> SRCTHLENRDFVTGTQGTTRVTLVLELGGCVTITAEGKPSMDVWLDAIYQENPAKTREYCLHAKLSDTKVAARCPTMGPATLAEEHQGGTVCKRDQSDRGWGNHCGLFGKGSIVACVKAACEAKKKATGHVYDANKIVYTVKVEPHTGDYVAANETHSGRKTASFTISSEKTILTMGEYGDVSLLCRVASGVDLAQTVILELDKTVEHLPTAWQVHRDWFNDLALPWKHEGAQNWNNAERLVEFGAPHAVKMDVYNLGDQTGVLLKALAGVPVAHIEGTKYHLKSGHVT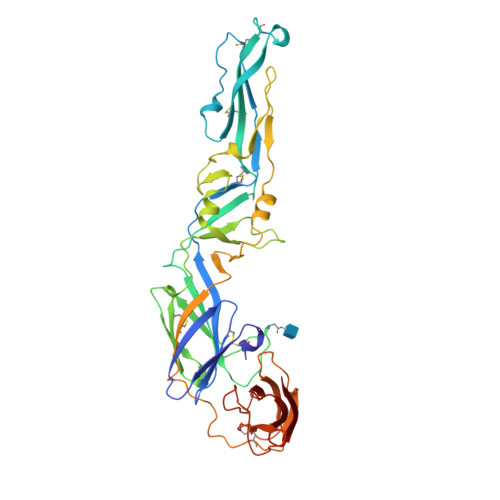CEVGLEKLKMKGLTYTMCDKTKFTWKRAPTDSGHDTVVMEVTFSGTKPCRIPVRAVAHGSPDVNVAMLITPNPTIENNGGGFIEMQLPPGDNIIYVGELSHQWFQK> PNLPQSVVGT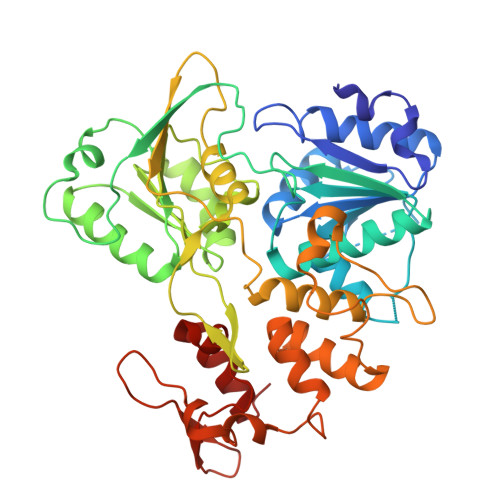GWTAKGQITVLDMHPGSGKTHRVLPELIRQCVERRLRTLVLAPTRVVLREMERALSGKNVRFHSPAVTEQHANGAIVDVMCHATYVNRRLLPQGRQNWEVAIMDEAHWTDPHSIAARGHLYSLAKENRCAFVLMTATPPGKSEPFPESNGAIASEERQIPDGEWRDGFDWITEYEGRTAWFVPSIARGGAIARALRQRGKSVICLNSKTFDKEYSRVKDEKPDFVVTTDISEMGANLDVTRVIDGRTNIKPEEVDGRIELTGTRRVTTASAAQRRGRVGRQGGRTDEYIYSGQCDDDDSGLVQWKEAQILLDNITTARGPVATFYGPEQERMTETAGHYRLPEEKRKHFRHLLAQCDFTPWLAWHVAANVASVTDRSWTWEGPEENAVDENNGELVTFRSPNGAERTLRPVWRDARMFREGRDIREFVSYASGRR> GSHMPETETEVTPIQQLFLIKELKPGIARIGVIWDKNAANRDEVLPQLQRASAATGIKVVVAEVASLQEVAPQFRTLLRDHQVEALWVLEESGLLGQAAARSFLIKNATQAGMPVFAPSETWLKEGACVTWRKDAEGIR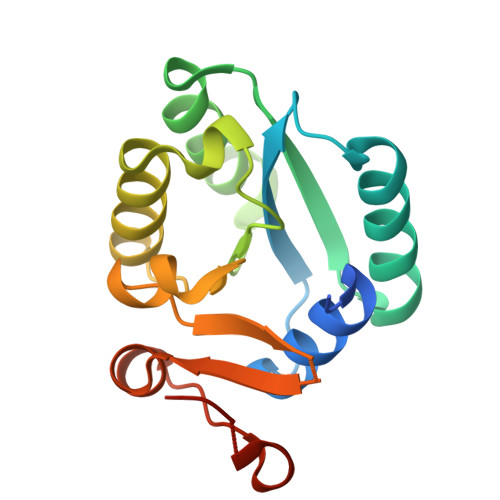LVVNKAVAEAMGITIPAKYQDRTAFLAMN>[2x]GAMPVTTPTKMATLTTKQMWQTIKDYFGDGFVTGSAPISYNVHTCDMQLQPDSGIHAASDGIHYGVQISEDSMPLFSIMGDTAAPPCTCHRVDEIVKHIDEFLERAPEALPDDGAITSGKPCDTNPDQVSLYAMRDSLSWWVHWGGNLRPEHYWKQIYIGFAAIPDDVQISPREFLDGTYR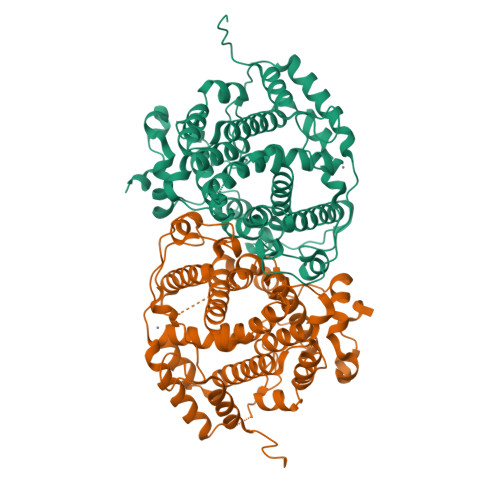YLGHTWDDCLSGLEEEGVSPDEIEFANMCMWRQMLTQWLEKADPELLPLLKGKISLMLQYRVLTANTLGCLALFMNATADPKDGPIHYADSSYEMEIASVAQCVTLDMAKEAMGILQGERTEVVAGDRAQRKRELRWIYVRCMQILESQPHAHMLRRYGSAGLHYVPMMDRYLERVSGHTRFPIRDGAARILERFINRAELPKESEDINPNGRSLKVSAKMNGNGQLHHEVNGNAKLHLEAERPDVTTAVG> GSHMVPISFVFNRFPRMVRDLAKKMNKEVNFIMRGEDTELDRTFVEEIGEPLLHLLRNAIDHGIEPKEERIAKGKPPIGTLILSARHEGNNVVIEVEDDGRGIDKEKIIRKAIEKGLI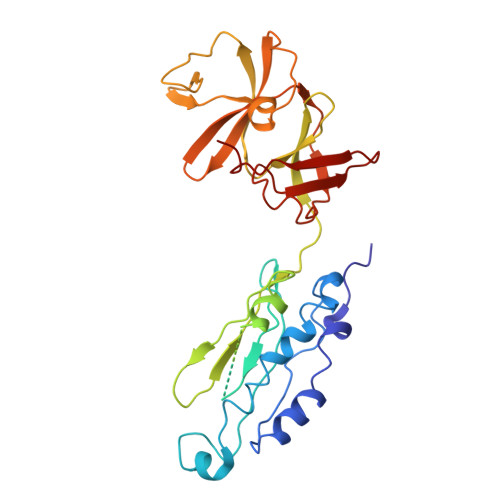DESKAATLSDQEILNFLFVPGFSTKEKVSEVSGRGVGMDVVKNVVESLNGSISIESEKDKGTKVTIRLPLTLAIIQALLVKVNNLVYAIPIANIDTILSISKEDIQRVQDRDVIVIRGEVIPVYRLWEVLQIEHKEELEEMEAVIVRVGNRKYGIVVDDLLGQDDIVIKSLGKVFSEVKEFSGAAILGDGSIALIINVSGIV>[2x]GAHMGGSMSYQVLARKWRPQTFADVVGQEHVLTALANGLSLGRIHHAYLFSGTRGVGKTSIARLLAKGLNCETGITATP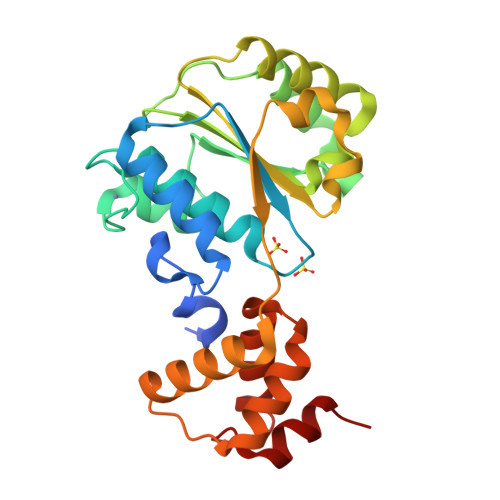CGVCDNCREIEQGRFVDLIEIDAASRTKVEDTRDLLDNVQYAPARGRFKVYLIDEVHMLSRHSFNALLKTLEEPPEHVKFLLATTDPQKLPVTILSRCLQFHLKALDVEQIRHQLEHILNEEHIAHEPRALQLLARAAEGSLRDALSLTDQAIASGDGQVSTQAVSAMLGT>APDWVPPEVFDLVAEDKARCMSEHGTTQAQIDDVDKGNLVNEPSITCYMYCLLEAFSLVDDEANVDEDIMLGLLPDQLQERAQSVMGKCLPTSGSDNCNKIYNLAKCVQES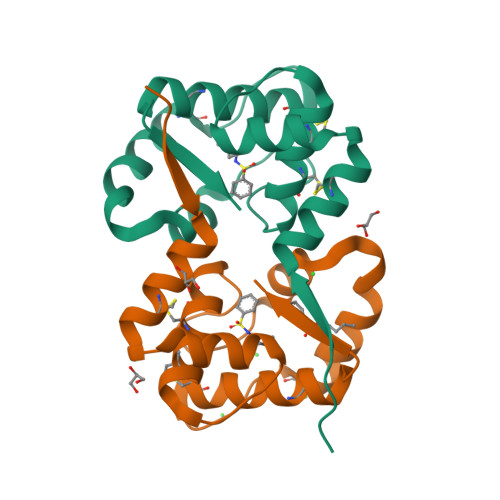APDVWFVI[2x]> GYFEGMLIKQTDYFRIYRVINSLLISQNADPASASMYFSTFGAFILQQHYKVKAVPKGGLAAYNLGGTVLLFADHREDGYVTGAGENFHCWVEADGWAIDFMAPAFSEGTDALAVPAKMFQRPLSAMAASINDLGQSGDFFYRSEPEATARRFADWHKQAMIGDMASVAANWFRKSPKQMAASLS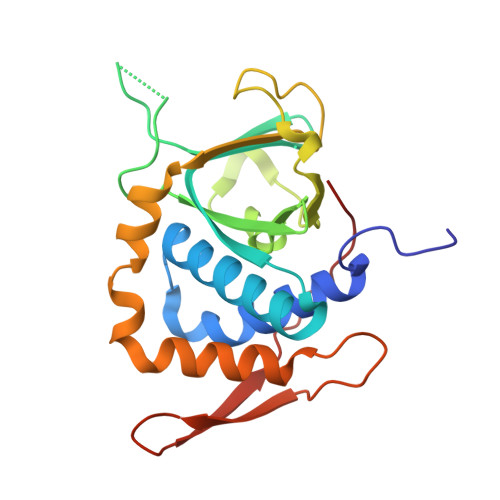VTDRDGKARTVPLTGEMLTGAW> RDPVPTQGYRVVKRYPHDTTAFTEGLFYLRGHLYESTGETGRSSVRKVDLETGRILQRA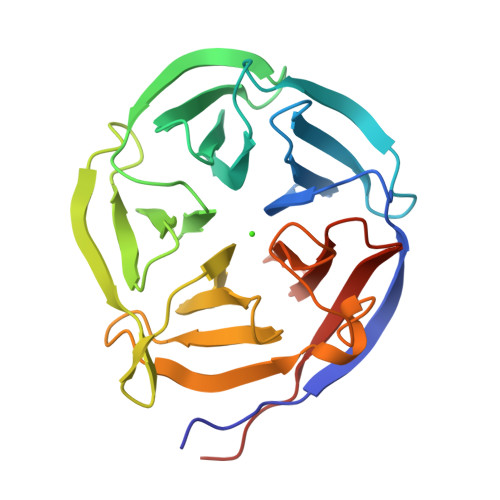EVPPPYFGAGIVAWRDRLIQLTWRNHEGFVYDLATLTPRARFRYPGEGWALTSDDSHLYMSDGTAVIRKLDPDTLQQVGSIKVTAGGRPLDNLNELEWVNGELLANVWLTSRIARIDPASGKVVAWIDLQALVPDADALTDSTNDVLNGIAFDAEHDRLFVTGKRWPMLYEIRLTPLPHAAAGK> DCSSSWSSYEGHCYKAFKQSKTWADAESFCTKQVNGGHLVSIESSGEADFVAHLIAQKIKSAKI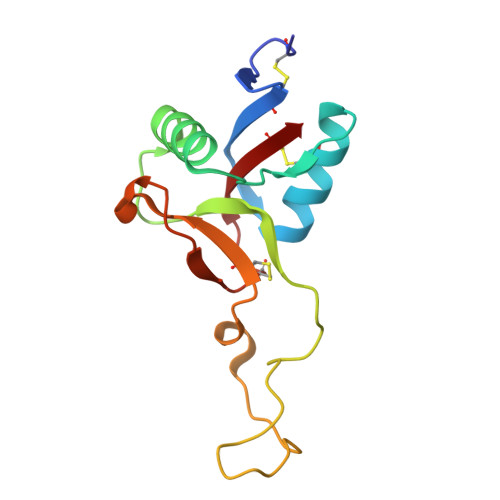HVWIGLRAQNKEKQCSIEWSDGSSISYENWIEEESKKCLGVHKATGFRKWENFYCEQRDPFVCEA> GSFTESNNQTQDFERAAKKLSQKEINRRMALAQAYNDSLNNVHLEDPYEKKRIQKGIAEYARMLEVSEKIGIISVPKIGQKLPIFAGSSQEVLSKGAGHLEGTSLPIGGNSTHTVITAHSGIPDKELFSNLKKLKKGDKFYIQNIKETIAYQVDQIKVVTPDNFSDLLVVPGHDYATLLTCTPIMV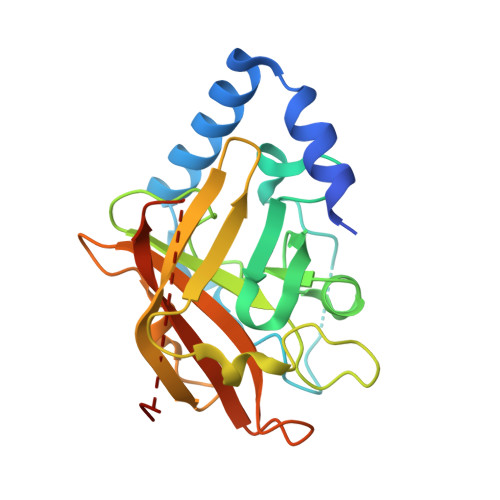NTHRLLVRGHRIPYKGPIDEKLIKDGHLNT>MNYEGKTKIVKVTGDYALLEFKDDITAGDGLKHDVLTGKGSICAETTAILMKYLSEKGIKTHLVEYIPPRTLKVIPLKMFPLEVVVRLKKAGSFVRRYGGAEGEDLPVPLVEFFIKDDERHDPMVCVDHLEILGIATKKQAEKMKEAAVKITLALKEFFERANFELWDIKYEFGLDKDGNVVLGDEI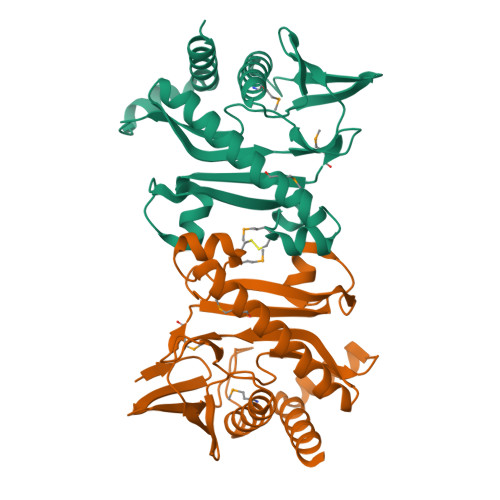SPDTFRLRKKGEIFDKDVYRRDLGDPLKKYREVLELCRSLNSQ[2x]>MSLEAAGGIVWRWKAGSDIANDPAIASSKSAQEQLDSIEVCIVHRPKYDDWSWPKGKLEQNETHRHAAVREIGEETGSPVKLGPYLCEVEYPLSEEGKKTRHSHDCTADTKHTLYWMAQPISADDAEHLLDAFGPVHRADVGEINDIVWVSVREARKILSHSTDKDTLAVFVDRVQEGAATAQNLLIVRHAKAESRKSWKGTDANRPITPKGAAMAFALNRELACFNPTRLATSPWLRCQET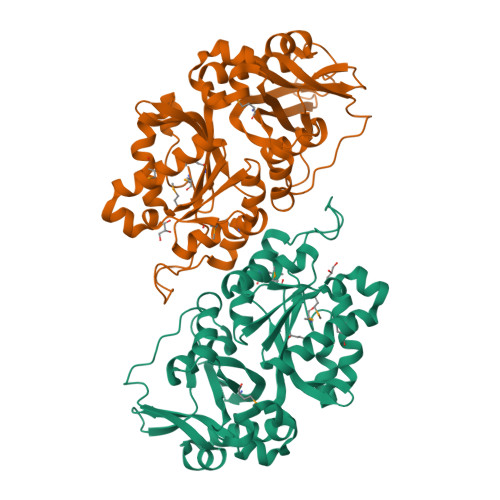LQVLSWQTERPMEHINTLTEDAFAEHPAVSWLAFREQITQTLNSRETTAICMHRPVIGGMYDHLRGLCARKQLAKQLIAKSPYMPTGTAMSLFIIDTPQGPSIIDIQKVSPIVYEGHHHHHH[2x]> MDIAQDWNGIPVPANPGNGMTWQLQDNVSDSFNYTSSEGNRPTAFTSKWKPSYINGWTGPGSTIFNAPQAWTNGSQLAIQAQPAGNGKSYNGIITSKNKIQYPVYMEIKAKIMDQVLANA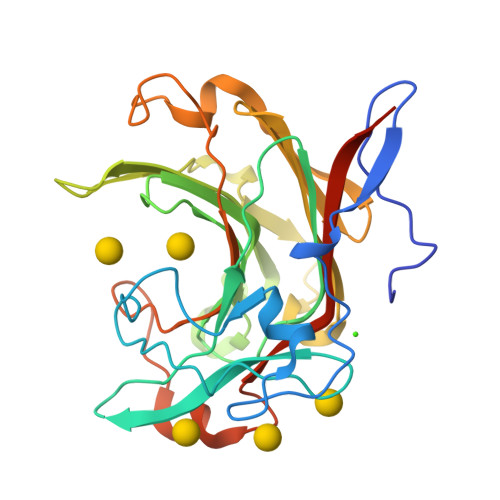FWTLTDDETQSIDIMEGYGSDRGGTWFAQRMHLSHHTFIRNPFTDYQPMGDATWYYNGGTPWRSAYHRYGCYWKDPFTLEYYIDGVKVRTVTRAEIDPNNHLGGTGLNQATNIIIDCENQTDWRPAATQEELADDSKNIFWVDWIRVYKPVAVSLEHHHHHH> MGYVGIKIRLTDVAPQAQELFKKESLDVKENKVYLVAATLRPETMYGQTCCFVSPKIDYGVFDAGNGDYFITTERAFKNMSFENLTPERGYYKPLFTINGKTLIGSRIDAPYAVNKNLRVLPMETVLATKGTGVVTCVPSDSPDDFVTTRDLANKPEYYGIEKDWVQTDIVPIVHTEKYGDKCAEFLVNDLKIQSPKDSVQLANAKELAYKEGFYNGTMLIGKYKGDKVEDAAPKVKQDLIDEGLAF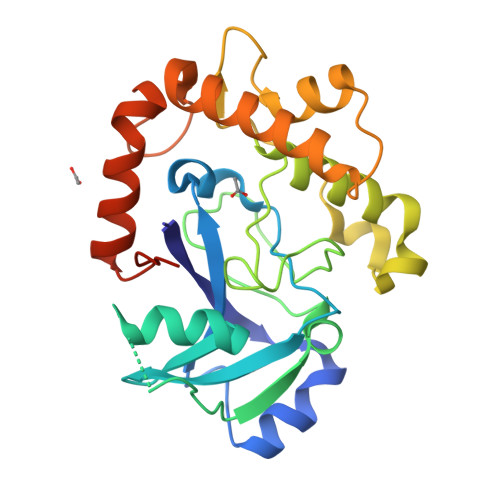VYNEPELEHHHHHH> MQAQITGRPEWIWLALGAALMGLGALYFLVKGMGVSDPDAKKFYAITALVPAI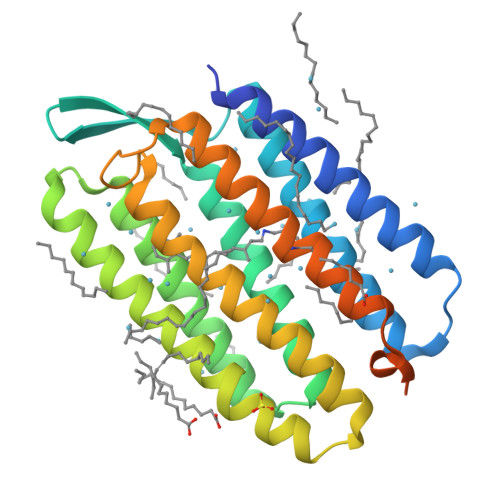AFTMYLSMLLGYGLTMVPFGGEQNPIYWARYADWLFTTPLLLLDLALLVDADQGTILALVGADGIMIGTGLVGALTKVYSYRFVWWAISTAAMLYILYVLFFGFTSKAESMRPEVASTFKVLRNVTVVLWSAYPVVWLIGSEGAGIVPLNIETLLFMVLDVSAKVGFGLILLRSRAIFGEAEAPEPSAGDGAAATSDGSGIEGRSGAPHHHHHHHH> GANSVLFPCKYASSGCEITLPHTEKADHEELCEFRPYSCPCPGASCKWQGSLDAVMPHLMHQHKSITTLQGEDIVFLATDINLPGA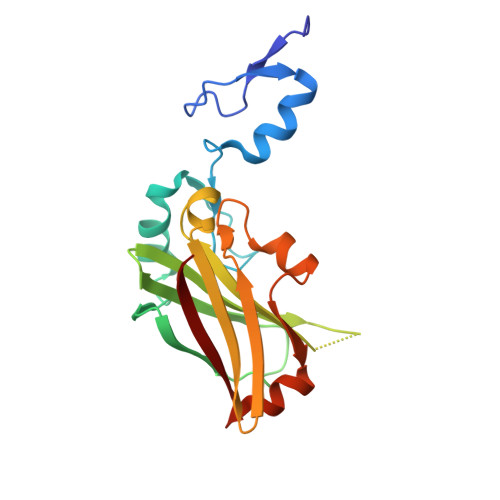VDWVMMQSCFGFHFMLVLEKQEKYDGHQQFFAIVQLIGTRKQAENFAYRLELNGHRRRLTWEATPRSIHEGIATAIMNSDCLVFDTSIAQLFAENGNLGINVTISMC>MLDEKSSNTAVVVVLCTAPDEATAQDLAAKVLAEKLAACATLIPGATSLYYWEGKLEQEYEVQMILKTTVSHQQALLECLKSHHPYQTPELLVLPVTHGDTDYLSWLNASL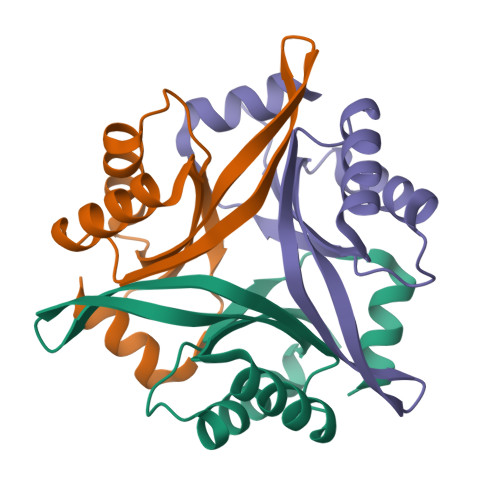R[6x]3-BROMOBUT-3-EN-1-OL | C4 H7 Br 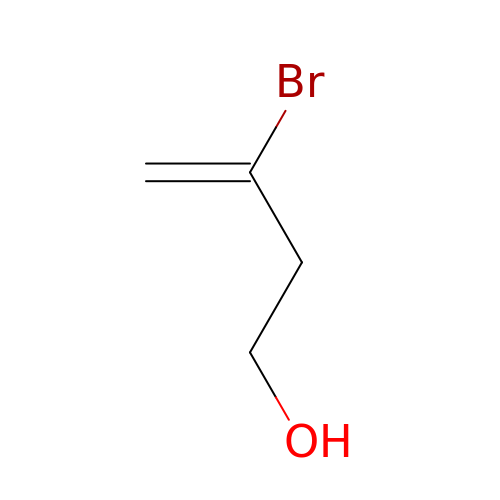O | RTKMFQOHBDVEBC-UHFFFAOYSA-N4-butoxy-3-chlorobenzyl imidothiocarbamate | C12 H17 Cl N2 O S | 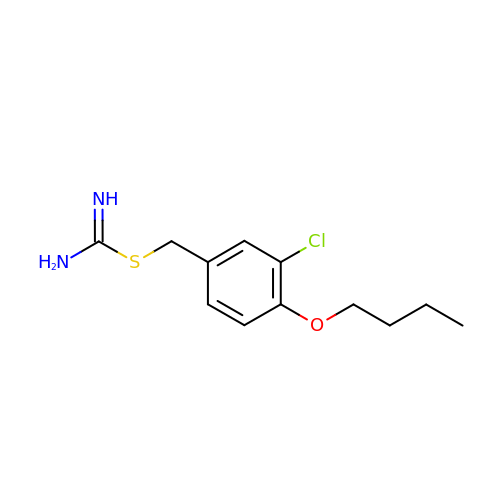IONZMLSFEITLRK-UHFFFAOYSA-N> MIAYDITPIDLHGHLFNVSLTIEQTNDEQELWLPNWIPGSYLIRDFSKHIIGLHAESNGLSLPVKQISKNRWQLARSKHPVTVHYQVYAWDLSVRSAYLDQFQGFFNNTSLCLAVEGQTDLPCELHLHAPPEAPLWKVATGMPRKSGQPHSWGCFRADNYDALIDYPFLIGDLT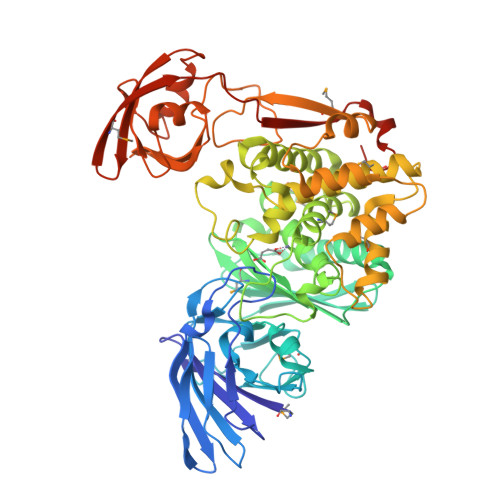IEEFIAHGIKHSLVLSGRHYADTSRITADLAKICETQISLFEEAPFQSYTFLTMVVGNGFGGLEHRNSTALLCSRKDLISAHQYEMNDNYQTFLSLCCHEYFHSWNIKTLKPKAFLPYQLEKESYTEQLWFYEGMTSYFDDYLLHTSGIIDEKRYLKLLGDTLSRVERGAGQYQQSVTESSFLAWTKFYQQNENAPNSIVSYYAKGALIALSLDLMLRLQSDHKLTLARVMKELWHEFGKTSIGTADDTVINWLNQYPGIDISDFLKDALYNKESLSLVELLQNFGVMVQKQVPVDDNSVGGKASEQPARVNFGAKYKASPQGLDVLNVYHDESAYHAGLSAGDKIIAIDHLQATEQSVKRILERYIPGDTVTIHAFRRDELMTLELTWQEPAKSSYVLSVEQPDKLKGWLTPSGLEHHHHHH>I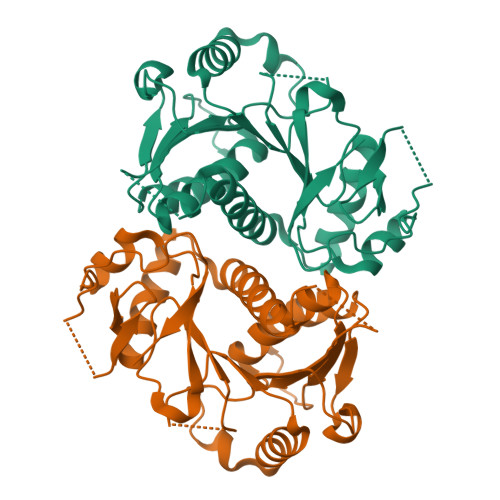LESEPIVYRRIIVPHNVSKEFCTDSGLVVPSISYELHKKLLSVAEKHGLTLERRLEMTGVCASQMALTLLGGPNRLNPKNVHQRPTVALLCGPHVKGAQGISCGRHLANHDVQVILFLPNFVKMLESITNELSLFSKTQGQQVSSLKDLPTSPVDLVINCLDCPENVFLRDQPWYKAAVAWANQNRAPVLSIDPPVHEVEQGIDAKWSLALGLPLPLGEHAGRIYLCDIGIPQQVFQEVGINYHSPFGCKFVIPLHSA[4x]> TRDQNGTWEMESNENFEGYMKALDIDFHTRKIAVRLTQTKVIDQ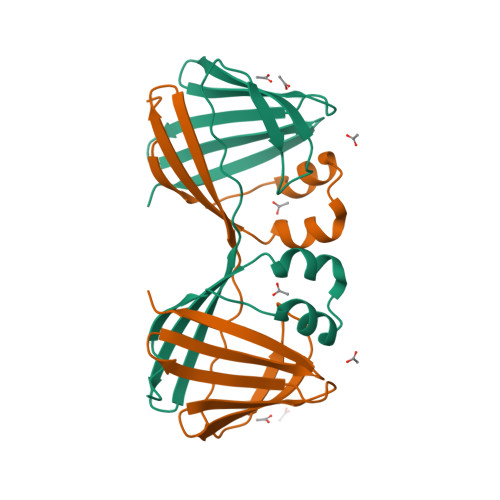DGDNFKDKTTSTFRNYDVDFTVGVEFDEYTKSLDNRHVKALVTWEGDVLVCVQKGEKENRGWKKWIEGDKLYLELTCGDQVCRQVFKKK> GPRKQRKDYEEGE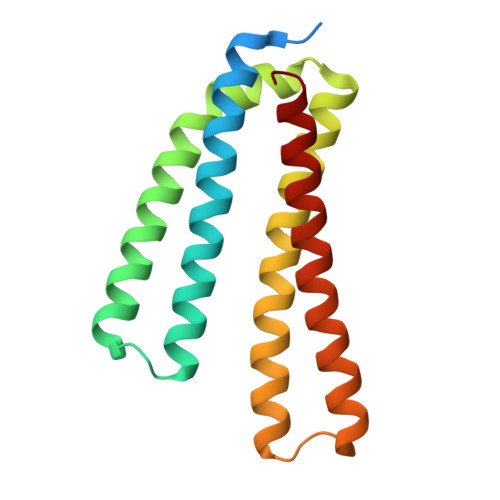ESFIEQSVPIRELTRFVTLIEEKNAILLDIEKADSDLRRKRIQKKVYTKTVKNYQNKLKELNEESIPFKRILMETGGQIQSIIQKLDFLEAEKISVKDSVKLLKDRYKRGKLPSKAAYERLSSDMIKQLASSQNKIDRYINELRAYII>MKFAEHLSAHITPEWRKQYIQYEAFKDMLYSAQDQAPSVEVTDEDTVKRYFAKFEEKFFQTCEKELAKINTFYSEKLAEAQRRFATLQNELQSSLDAQKESTGVTTLRQRRKPVFHLSHEERVQHRNIKDLKLAFSEFYLSLILLQNYQNLNFTGFRKILKKHDKILETSRGADWRVAHVEVAPFYTCKKINQLISETEAVVTNELEDGDRQKAMKRLRVPPLGAAQPAPAWTTFRVGLFCGIFIVLNITLVLAAVFKLETDRSIWPLIRIYRGGFLLIEFLFLLGINTYGWRQAGVNHVLIFELNPRSNLSHQHLFEIAGFLGILWCLSLLACFFAPISVIPTYVYPLALYGFMVFFLINPTKTFYYKSRFWLLKLLFRVFTAPFHKVGFADFWLADQLNSLSVILMDLEYMICFYSLELKWDESKGLLPNNSEESGICHKYTYGVRAIVQCIPAWLRFIQCLRRYRDTKRAFPHLVNAGKYSTTFFMVTFAALYSTHKERGHSDTMVFFYLWIVFYIISSCYTLIWDLKMDWGLFDKNAGENTFLREEIVYPQKAYYYCAIIEDVILRFAWTIQISITSTTLLPHSGDIIATVFAPLEVFRRFVWNFF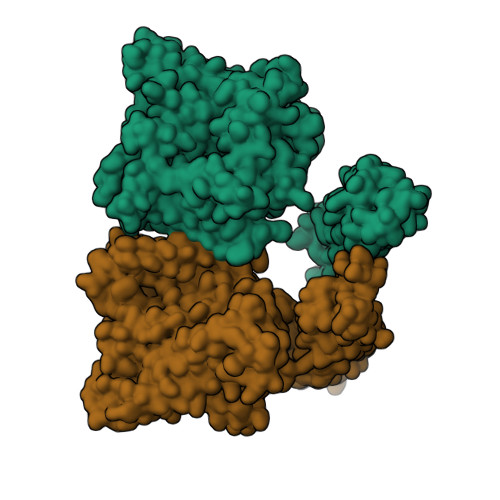RLENEHLNNCGEFRAVRDISVAPLNADDQTLLEQMMDQDDGVRNRQKNRSWKYNQSISLRRPRLASQSKARDTKVLIEDTDDEANT[2x]3-(4-aminocarbonylphenyl)benzoic 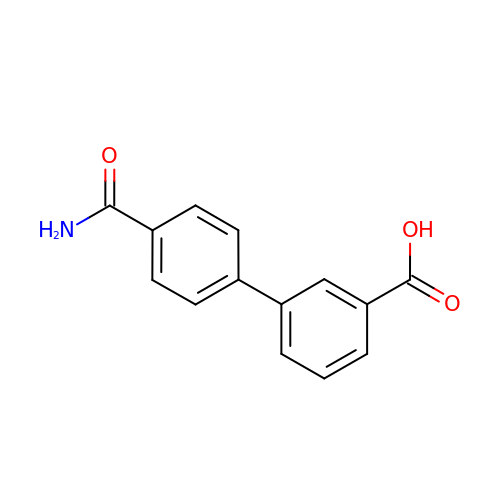acid | C14 H11 N O3 | NZYMBNSXWYJPEG-UHFFFAOYSA-N>[2x]MVMKQTKQTNILAGAAVIKVLEAWGVDHLYGIPGGSINSIMDALSAERDRIHYIQVRHEEVGAMAAAADAKLTGKIGVCFGSAGPGGTHLMNGLYDAREDHVPVLALIGQFGTTGMNMDTFQEMNENPIYADVADYNVTAVNAATLPHVIDEAIRRAYAHQGVAVVQIPVDLPWQQIPAEDWYASANSYQTPLLPEPDVQAVTRLTQTLLAAERPLIYYGIGARKAGKELEQLSKTLKIPLMSTYPAKGIVADRYPAYLGSANRVAQKPANEALAQADVVLFVGNNYPFAEVSKAFKNTRYFLQIDIDPAKLGKRHKTDIAVLADAQKTLAAILAQVSERESTPWWQANLANVKNWRAYLASLEDKQEGPLQAYQVLRAVNKIAEPDAIYSIDVGDINLNANRH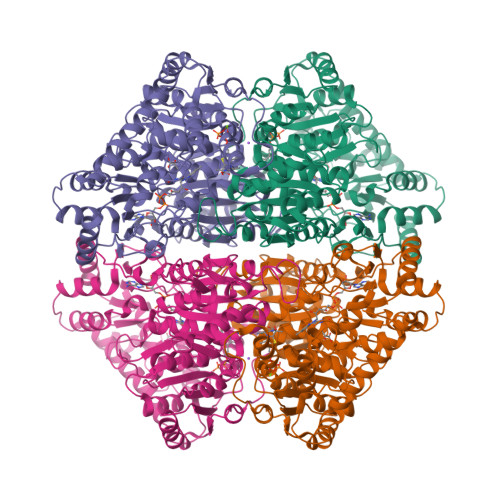LKLTPSNRHITSNLFATMGVGIPGAIAAKLNYPERQVFNLAGDGGASMTMQDLATQVQYHLPVINVVFTNCQYGWIKDEQEDTNQNDFIGVEFNDIDFSKIADGVHMQAFRVNKIEQLPDVFEQAKAIAQHEPVLIDAVITGDRPLPAEKLRLDSAMSSAADIEAFKQRYEAQDLQPLSTYLKQFGLDDLQHQIGQGGF>GSLDKWEMERTDITMKHKLGGGQYGEVYEGVWKKYSLTVAVKTLKEDTMEVEEFLKEAAVMKEIKHPNLVQLLGVCTREPPFYIIIEFMTYGNLLDYLRECNRQEVSAVVLLYMATQISSAME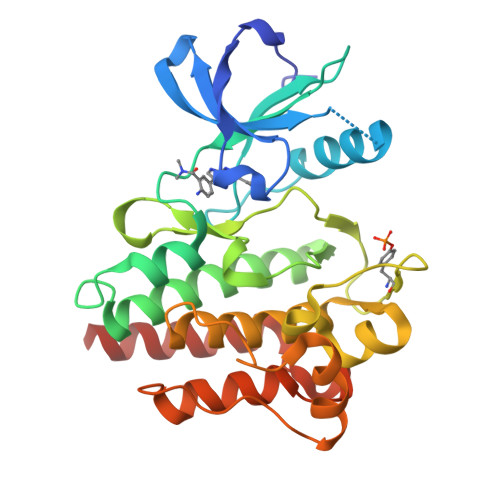YLEKKNFIHRDLAARNCLVGENHLVKVADFGLSRLMTGDTYTAHAGAKFPIKWTAPESLAYNKFSIKSDVWAFGVLLWEIATYGMSPYPGIDPSQVYELLEKDYRMERPEGCPEKVYELMRACWQWNPSDRPSFAEIHQAFETMFQESSISDEG[2x]> PITLVKDILSKPPITAHSNISIMEAAKILIKHNINHLPIVDEHGKLVGIITSWDIAKALAQNKKTIEEIMTRNVITAHEDEPVDHVAIKMSKYNISGVPVVDD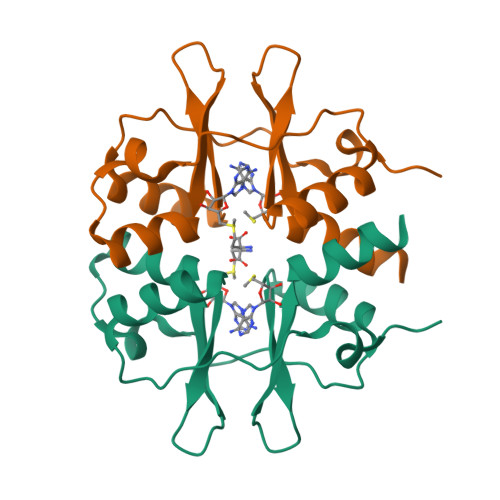YRRVVGIVTSEDISRLFGGKK Integration into host target DNA (tDNA), a hallmark of retroviral replication, is mediated by the intasome, a multimer of integrase (IN) assembled on viral DNA (vDNA) ends. Integration is mediated by the viral integrase (IN) protein, which catalyzes sequential 3′-processing and strand transfer reactions. Retroviral INs are composed of three canonical structural domains: an α-helical N-terminal domain (NTD), the catalytic core domain (CCD, which adopts an RNase H-like fold and harbors the enzyme active site), and the C-terminal domain (CTD, featuring an SH3-like β-barrel fold). Simiispumaviruses, typified by PFV, as well as δ-retroviruses that include human lymphotropic virus 1 (HTLV-1), employ four IN molecules, while α-retroviruses and β-retroviruses, the latter of which include mouse mammary tumor virus (MMTV), use eight.

We have accordingly determined the structure of the MMTV STC resolved to 3.5 Å resolution, with more acute 3 Å resolution in the intasome core region. To recapitulate the TSD observed in MMTV infected cells, we assembled MMTV STCs using a bDNA that harbored two vDNA ends covalently joined to opposing tDNA 5'-phosphates separated by 6 bp. As previously done for the MMTV CSC, Ca2+, which can enhance specific IN-vDNA interactions without supporting IN catalytic function, was included to enhance STC assembly. As observed for the MMTV CSC intasome, the STC complex comprises eight IN molecules. The central region includes four CTDs emanating from the flanking dimers (two from each side) and four IN protomers in which all domains are constrained to the core region. The latter can be subdivided into two inner INs that perform the catalytic cleavage reactions, which in the STC contact both vDNA and tDNA, and two outer INs that are not involved in catalysis. The structure revealed a pronounced bend in tDNA, which transitions from B-form DNA in peripheral regions to the A-form in and around the sites of vDNA joining. In comparison to the vDNA or to the peripheral regions of tDNA, which maintain ∼16 Å phosphate-phosphate distances in the major grooves, the tDNA major groove begins to noticeably widen at bp positions –1/+6, reaching a maximum distance of ∼22 Å within the central two dinucleotides of the cleavage site. The tDNA configuration in and around the 6-bp cleavage site exhibits multiple characteristics of A-form DNA. CCD residue Pro125 makes base-specific contacts with tDNA bases at positions −3/+8, and Tyr149 inserts into the tDNA major groove, contacting bp positions −1/+6 and −2/+7. Pro125 and Tyr149 reside on opposite sides of the phosphate backbone, immediately adjoining each of the two tDNA cleavage sites, clasping the cleaved tDNA strand.

>[4x]ALESAQESHALHHQNAAALRFQFHITREQAREIVKLCPNCPDWGHAPQLGVNPRGLKPRVLWQMDVTHVSEFGKLKYVHVTVDTYSHFTFATARTGEATKDVLQHLAQSFAYMGIPQKIKTDNAPAYVSRSIQEFLARWKISHVTGIPYNPQGQAIVERTHQNIKAQLNKLQKAGKYYTPHHLLAHALFVLNHVNMDNQGHTAAERHWGPISADPKPMVMWKDLLTGSWKGPDVLITAGRGYACVFPQDAESPIWVPDRFIRPFTERKEATPTPGTAEKTPPRDEKDQQESPKNESSPHQREDGLATSAGVDLRSGGGP>MMFGSTKPESGDSKWRSQLDRFVKENQQDLAALFWGLWLENGDSQG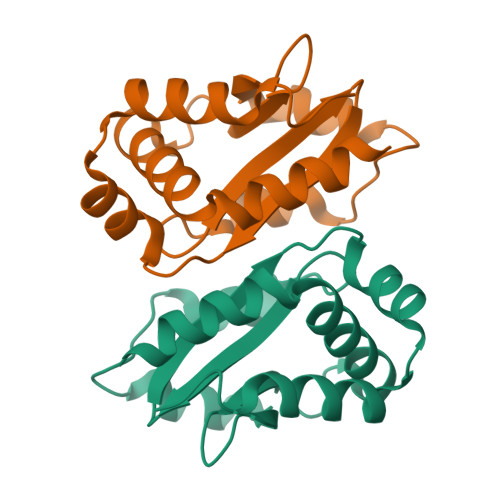TIGIDLQPTPHFVYCPKDAVEKLNNNVENRLQELLGIIEHNQPEIEVLMIGIGKGEIKLIQFAPEPPPPVCFEQVGKDIDGLLELLEQRMSGEIVV[2x]>[2x]MAHHHHHHMTTPRTTLITGAAGGIGQALVRRFLAAGDRVLALDRDRAALAAFVDALGGAAVAPVVDDLTDAARLADALANERVDVLVANAGTAASATLRATTSASWRADLDANLTATYVSVEAVLAGMRARRRGAITIVGSVNGVAALGHPAYSAAKAGLISYAKSLAIEYGRDGVRANVVCPGTVKTPAWEARVRQNPQVFEQLK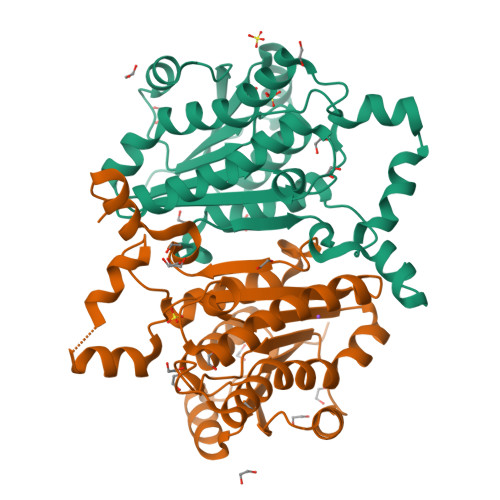KWYPLDDFATPDDVANAALFLSSDAARAITGAMLPVDGGLLAGNRVMAQELTLESFY>MGFDEKREPTGGRLRLQDIPALTQDHCRMRDPAEVERIINEFVIGGPERMQIVSDFDYTITKQRTEDGGAVPSSFGIFNACQSLPENFKAETDKLYHKYRPIEIDPHMPIAEKVQYMIEWWTKSGELTSGFPFDQSEIDQIASKYTHALRDRTHEFFADLQRLGIPTLVFSAGLGNSVVSVLRQANVLHPNVKVVSNFLQFRDGLLDGFQQPMIHTFNKNETVLNETSEYYDLVHTRDHIIVMGDSIGDADMASGVPASSHIMKIGFLFDHVEANMKKYMDTFDIVLVDDQTMDVPRTLLSLIEKQHKLNLEAPKQSSL[2x]

Although the intracellular 5′-nucleotidases generally share a low sequence similarity, all enzymes are magnesium-dependent and belong to the haloacid dehalogenase (HAD) superfamily. They are characterized by a modular architecture, containing a structurally conserved HAD core domain, which contains the catalytic residues, and an enzyme-specific cap domain consisting of one or more cap insertions. To gain insight into the broad substrate specificity of cN-IIIB and especially its unusual preference for m7GMP, we determined crystal structures of Drosophila melanogaster cN-IIIB (DmcN-IIIB) bound to different reaction products. The overall structure of DmcN-IIIB is similar to cN-IIIA, however, critical residues conferring substrate specificity and determining the size of the substrate-binding pocket are different.

DmcN-IIIB was crystallized in the presence of the reaction products 7-methylguanosine (m7G) or cytidine, and a mixture of AlCl3 and NaF. The structure model of DmcN-IIIB bound to m7G was refined at a resolution of 1.65 Å to R and Rfree values of 15.9% and 19.4%, respectively. The final model of the DmcN-IIIB m7G complex contains two molecules in the asymmetric unit with one continuous segment encompassing residues 13–311 of molecule A as well as residues 13–312 of molecule B, both superposing with a root mean square deviation (rmsd) of 0.86 Å for 288 common Cα atoms (residues 13–103 and 115–311). After all amino acids had been placed, additional density was observed in the active center, which, based on its shape, could be assigned as an octahedrally coordinated magnesium ion, the co-crystallized product nucleoside m7G as well as a metal fluoride transition state analog. It was shown that for pH values higher than 7.0, enzyme-MgF3 complexes rather than enzyme-AlF3 complexes are formed. The overall structure of DmcN-IIIB consists of two domains: the globular core domain and a smaller cap domain. The cap domain packs against the top of the HAD core and is composed of two regions, a C1-type cap (red) and a C2-type cap (blue). The co-crystallized reaction product 7-methylguanosine (m7G) is bound between the cap domain and the HAD core and is represented as stick model (carbon in yellow, nitrogen in blue, oxygen in red). Moreover, the slightly higher affinity of human cN-IIIB for m7GMP compared to DmcN-IIIB could be explained by the fact that one of the stacking residues in the Drosophila protein, Phe75, is replaced by a tyrosine (Tyr60) in the human counterpart.XANTHOSINE-5'-MONOPHOSPHATE 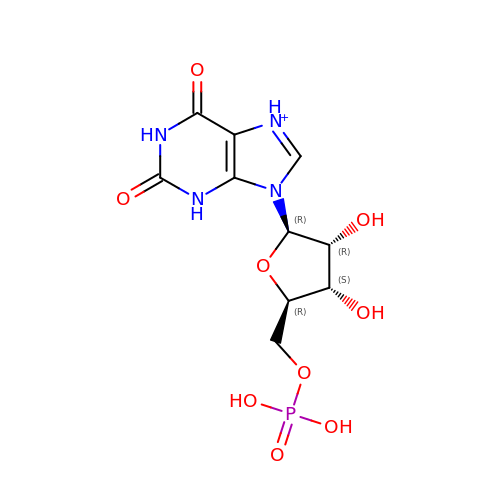| C10 H14 N4 O9 P | DCTLYFZHFGENCW-UUOKFMHZSA-O> MQQDRTYRHHGPEVSGWFSEQLMTGKIPLTEVFVDVENKPSPAPITIISGIVRQ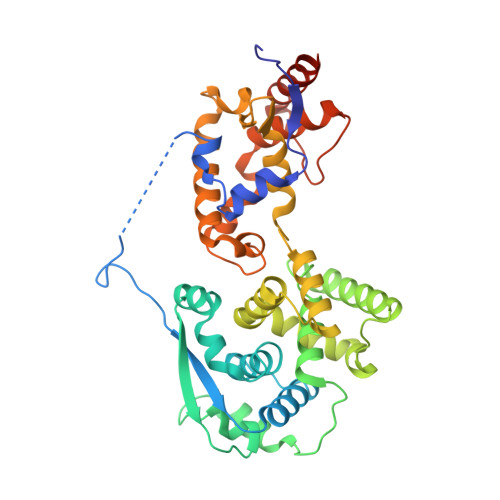RVIPVYVVNDLEGICQHIIQAFEAGVDFQDNADSFLLLLCLHHAYQGDHRLFLKSDAVQYLEGHGFRFEVREKENVHRLDELLPNVTGGKNLRRTLAAMPEEETTEANAGQFLSFASLFLPKLVVGEKACLEKVQRQIQVHAEQGLIQYPTSWQSVGHMMVIFRLMRTNFLIKFLLIHQGMHMVAGHDANDTVISNSVAQARFSGLLIVKTVLDHILQKTDLGVRLHPLARTAKVKNEVSSFKAALGSLAKHGEYAPFARLLNLSGVNNLEHGLYPQLSAIALGVATAHGSTLAGVNVGEQYQQLREAATEAEKQLQQYAETRELDNLG2-[4-[(~{Z})-1,2-diphenylbut-1-enyl]phenoxy]-~{N}-methyl-ethanamine | C25 H27 N O | 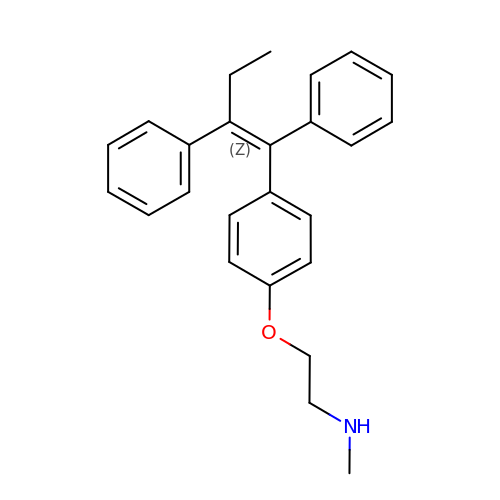NYDCDZSEEAUOHN-IZHYLOQSSA-N>HHHHHHMAEKKQWHETLHDQFGQYFAVDNVLYHEKTDHQDLIIFENAAFGRVMALDGVVQTTERDEFIYHEMMTHVPLLAHGHAKHVLIIGGGDGAMLREVTRHKNVESITMVEIDAGVVSFCRQYLPNHNAGSYDDPRFKLVIDDGVNFVNQTSQTFDVIISDCTDPIGPGESLFTSAFYEGCKRCLNPGGIFVAQNGVCFLQQEEAIDSHRKLSHYFSDVGFYQAAIPTYYGGIMTFAWATDNDALRHLSTEIIQAR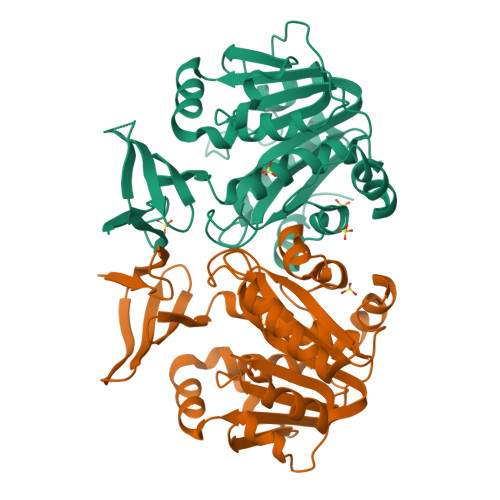FLASGLKCRYYNPAIHTAAFALPQYLQDALASQPS[8x]>[2x]MASPRKFFVGGNWKMNGDKAAIDGIISFMKTGPLSPNTEVVVGCPQCYLMYTREHMPANIGIAAQNCYKVAKGAFTGEISPAMVKDCGCEWVILGHSERRN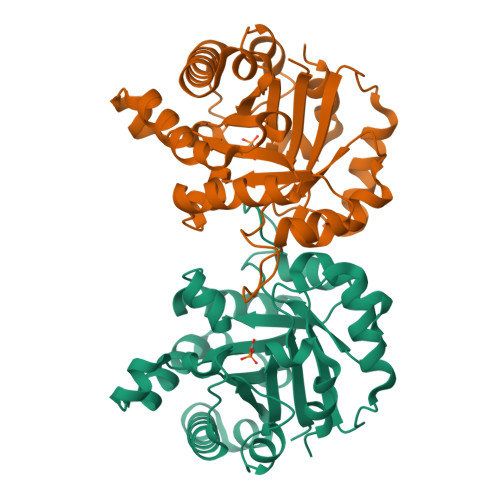VFGEPDQLISEKVGHALEAGLKVIPCIGEKLEDREGNRTQEVVFAQMKALLPNISDWSRVVLAYEPVWAIGTGKTASPEQAQEVHADLRQWLRDNVNAEVAESTRIIYGGSVSAGNCQELAKKGDIDGFLVGGAALKPDFVQIINARG>ADIVGAASPVTDAELYVAVGESQVNGGPHQAGKAGIGVGTVSNAKPVDFQGLSLYSGTTTVNGTAVRTLAMPITGAPGSHAGMGHFNFVKVG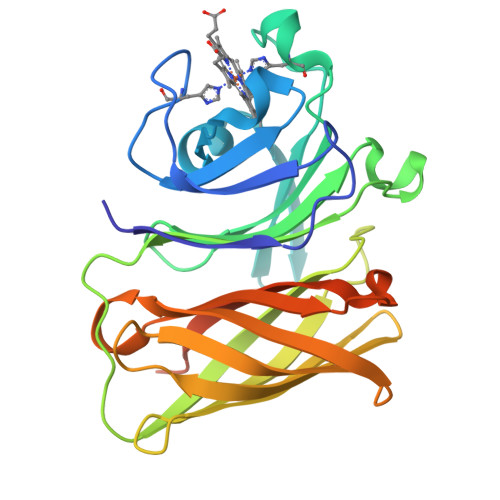SGDVWFGEWSKDGAAGGFNNRQVYFVGDRTGTTLPAGVATYSVAGLNKFNGSNLLSGTFRANFGSGTLQGGLTGGGLSVNVNASINSANASFAGSATANGTVAGTTQGQFFGANAATLAGIATFAGNSQYDTAFGGSKNELALVPRGSSAHHHHHHHHHH[2x]>SNASDKGKLSLQDVAELIRARACQRVVVMVGAGISTPSGIPDFRSPGSGLYSNLQQYDLPYPEAIFELPFFFHNPKPFFTLAKELYPGNYKPNVTHYFLRLLHDKGLLLRLYTQNIDGLERVSGIPASKLVEAHGTFASATCTVCQRPFPGEDIRADVMADRVPRCPVCTGVVKPDIVFFGEPLPQRFLLHVVDFPMADLLLILGTSLEVEPFASLTEAVRSSVPRLLINRDLVGPLAWHPRSRDVAQLGDVVHGVESLVELLGWTEEMRDLVQRET[4x]

Sirtuin 3 (SIRT3), a pivotal mitochondrial deacetylase, plays a critical role in restoring mitochondrial function, particularly through the activation of autophagy. The human SIRT3 protein contains a mitochondrial targeting sequence (MTS), an unstructured region and a conserved enzymatic core, which includes an NAD+ binding domain and a metal-binding motif. Sirtuins share a similar deacylation mechanism, with residue H248 being essential for their catalytic activity. SIRT3 regulates mitochondrial function by deacetylating, and thereby activating, numerous mitochondrial proteins involved in energy metabolism, oxidative stress responses, and cellular respiration.

Here, we report the identification of SKLB-11A, a SIRT3 activator with submicromolar affinity and high efficacy. In an effort to uncover the molecular interplay between SKLB-11A and SIRT3, we analyzed the structure of the SIRT3-SKLB-11A complex using X-ray crystallography at a resolution of 2.49 Å. The structural data revealed that the pyrrole ring of SKLB-11A inserts deeply into the cleft between two structural domains, where it forms a π-π stacking interaction with His248, a critical residue essential for deacetylase activity and conserved across the SIRT family (SIRT1–7). Furthermore, SKLB-11A formed a hydrogen bond with Val292 and tightly positioned between Phe180 and His248. Intriguingly, a significant conformational shift was observed in the side chain of Leu298, which deviated substantially from its orientation in previously reported SIRT3 structures. These findings suggest that SKLB-11A may modulate SIRT3 allosterically through an entirely novel mechanism. To further evaluate the functional consequences of side-chain reorientation, we substituted Leu298 with glycine. This mutation led to a marked reduction in enzymatic activity, as revealed by activity assays. Biochemical analysis further revealed a diminished binding affinity between SKLB-11A and the L298G mutant, with the dissociation constant increasing from 33.15 μM for the wild-type protein to 167.4 μM for the mutant. Collectively, these findings highlight the essential role of the Leu298 side chain in stabilizing the interaction between SKLB-11A and SIRT3 and preserving the enzyme’s deacetylase activity.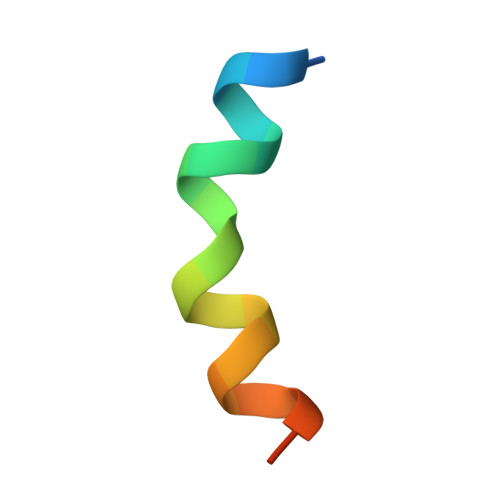> LNVKVLEALELYNKLVNEAPV>[2x]TTNKPIVLSTWNFGLHANVEAWKVLSKGGKALDAVEKGVRLVEDDPTERSVGYGGRPDRDGRVTLDACIMDENYNIGSVACMEHIKNPISVARAVMEKTPHVMLVGDGALEFALSQGFKKENLLTAESEKEWKEWLKTSQYKPIVNIENHD;>[2x]CIGM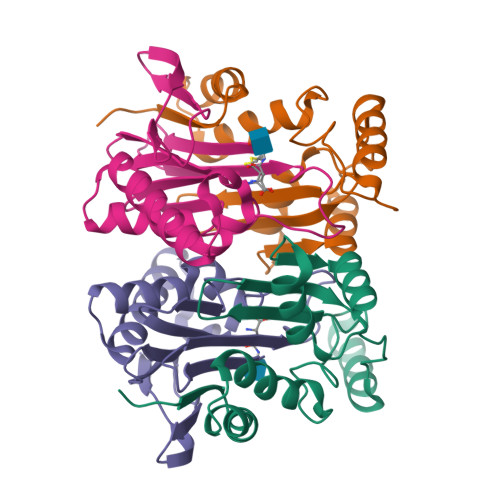IALDAQGNLSGACTTSGMAYKMHGRVGDSPIIGAGLFVDNEIGAATATGHGEEVIRTVGTHLVVELMNQGRTPQQACKEAVERIVKIVNRRGKNLKDIQVGFIALNKKGEYGAYCIQDGFNFAVHDQKGNRLETPGFALK> RLSGYCGSPWRVIGYHVVVWMMAGIPLLLFRWKPLWGVRLRLRPCNLAHAETLVIEIRDKEDSSWQLFTVQVQTEAVSVGQLEPSPQSQAEDGRSQAAVGAVPEGAWKDTAQLHKSEEAKRVLRYYLFQGQRYIWIETQQAFYQVSLLDHGRSCDDVHRSRHGLSLQDQMVRKAIYGPNVISIPVKSYPQLLVDEALNPYYGFQAFSIALWLADHYYWYALCIFLIS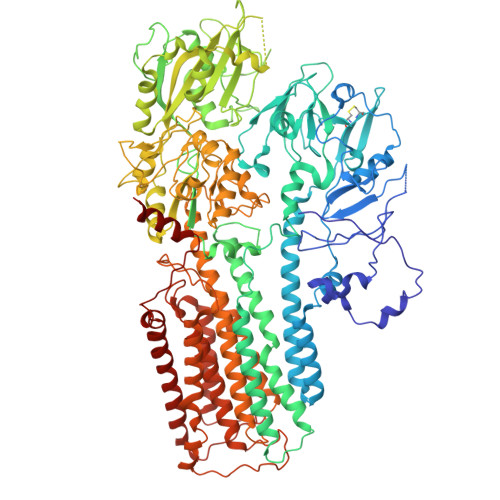SISICLSLYKTRKQSQTLRDMVKLSMRVCVCRPGGEEEWVDSSELVPGDCLVLPQEGGLMPCDAALVAGECMVNESSLTGESIPVLKTALPEGLGPYCAETHRRHTLFCGTLILQARAYVGPHVLAVVTRTGFCTAKGGLVSSILHPRPINFKFYKHSMKFVAALSVLALLGTIYSIFILYRNRVPLNEIVIRALDLVTVVVPPALPAAMTVCTLYAQSRLRRQGIFCIHPLRINLGGKLQLVCFDKTGTLTEDGLDVMGVVPLKGQAFLPLVPEPRRLPVGPLLRALATCHALSRLQDTPVGDPMDLKMVESTGWVLEEEPAADSAFGTQVLAVMRPPLWEPQLQAMEEPPVPVSVLHRFPFSSALQRMSVVVAWPGATQPEAYVKGSPELVAGLCNPETVPTDFAQMLQSYTAAGYRVVALASKPLPTVPSLEAAQQLTRDTVEGDLSLLGLLVMRNLLKPQTTPVIQALRRTRIRAVMVTGDNLQTAVTVARGCGMVAPQEHLIIVHATHPERGQPASLEFLPMESPTAVNGVKDPDQAASYTVEPDPRSRHLALSGPTFGIIVKHFPKLLPKVLVQGTVFARMAPEQKTELVCELQKLQYCVGMCGDGANDCGALKAADVGISLSQAEASVVSPFTSSMASIECVPMVIREGRCSLDTSFSVFKYMALYSLTQFISVLILYTINTNLGDLQFLAIDLVITTTVAVLMSRTGPALVLGRVRPPGALLSVPVLSSLLLQMVLVTGVQLGGYFLTLAQPWFVPLNRTVAAPDNLPNYENTVVFSLSSFQYLILAAAVSKGAPFRRPLYTNVPFLVALALLSSVLVGLVLVPGLLQGPLALRNITDTGFKLLLLGLVTLNFVGAFMLESVLDQCLPACLRRLRPKRASKKRFKQLERELAEQR>[4x]GPGSMVTSRLFALIPCAGTGSRSG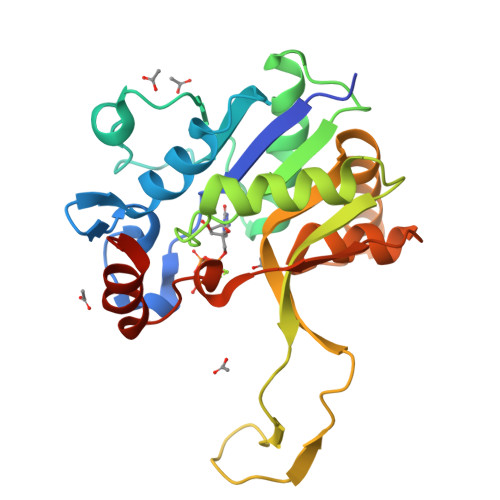SALPKQYRTLAGRALLHYTLAAFDACSEFAQTLVVISPDDAHFDARRFAGLRFAVRRCGGASRQASVMNGLIQLAEFGATDADWVLVHDAARPGITPALIRTLIGALKDDPVGGIVALPVADTLKRVPAGGDAIERTESRNGLWQAQTPQMFRIGMLRDAIQRAQLEGRDLTDEASAIEWAGHTPRVVQGSLRNFKVTYPEDFDLAEAILAHPARAS Bacterial AAA+ proteases are composed of a AAA+ partner (e.g., ClpC) and an associated peptidase (e.g., ClpP). They represent ATP-fuelled and self-compartmentalized proteolytic machines that are crucial for stress resistance and virulence. ClpC requires cooperation with adaptor proteins such as MecA for activation and complex formation with ClpP. Here, we present the cryo-EM structure of the MecA/ClpC/ClpP complex from the major pathogen Staphylococcus aureus.

The ClpP double heptamer was resolved at 2.7 Å overall resolution. ClpP is in the extended active conformation with the chamber gate, made of the seven β-hairpins, opened and all catalytic residues (S98, H123 and D172) correctly positioned. The pore formed by the β-hairpin collar is ~30 Å in diameter and is much less constrained compared to E. coli ClpP crystal structures, being ~15 Å51. As expected, while the ClpP part has an overall D7 symmetry with a very rigid core which can be refined to 2.7 Å resolution, the ClpC ATPase body deviates from a C6 symmetry that cannot really be applied and reaches an overall resolution of 2.9 Å in C1. Five out of seven ClpP β-hairpin NTDs (Pa-Pd, Pf) are fully visible from residues 1 to 28 while the β-hairpin loop T11-R16 is not visible in the ClpP subunits Pe and Pg. The ClpP hairpins also form stabilizing contacts between each other via T6, R13, G14, E15, R16 and additionally S22, a residue that is not part of the β-hairpin. These lateral ClpP β-hairpin contacts involve the loop of the hairpin for protomers Pa-Pf, while they shift toward the base of the β strand for the Pf-Pg-Pa interaction.

>[14x]MNLIPTVIETTNRGERAYDIYSRLLKDRIIMLGSQIDDNVANSIVSQLLFLQAQDSEKDIYLYINSPGGSVTAGFAIYDTIQHIKPDVQTICIGMAASMGSFLLAAGAKGKRFALPNAEVMIHQPLGGAQGQATEIEIAANHILKTREKLNRILSERTGQSIEKIQKDTDRDNFLTAEEAKEYGLIDEVMVPETK> MSRGSMEGQGCCGGGGGKTEMIPTEEALRIVFGVSKRLPPVIVSLYEALGKVLAEDIR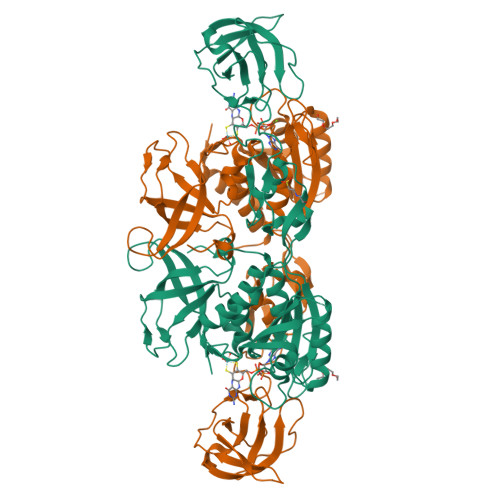APDPLPPYPASVKDGYAVVASDGPGEYPVITESRAGNDGLGVTVTPGTVAYVTTGGPIPDGADAVVQVEDTKVIGDVSTESKRVKILIQTKKGTDIRRVGCDIEKDATVLTTGERIGASEIGLLATAGVTMVKVYPMPIVAILSTGDELVEPTAGTLGRGQIRDSNRAMLVAAVMQQQCKVVDLGIVRDDRKELEKVLDEAVSSGVDIILTSGGVDMGDRSFVKPLLEEKGKVYFSKVLMKPGKPLTFAEIRAKPTESMLGKTVLAFGLPGNPVSCLVCFNIFVVPTIRQLAGWTSPHPLRVRLRLQEPIKSDPIRPEFHRAIIKWKDNDGSGTPGFVAESTGHQMSSRLLSMRSANALLELPATGNVLSAGSSVSAIIVSDISAFSIDKKASLSEPGSTSGGSAWSHPQFEK>[2x]GEIQWMKSNKETGRLNINGPTRTKLEPSAFYDVFEGSKKPAVLTSKDPRLEVDFEQALFSKYVGNTLHEPDEYVTQAALHYANQLKQLDINVNKMSMEEAC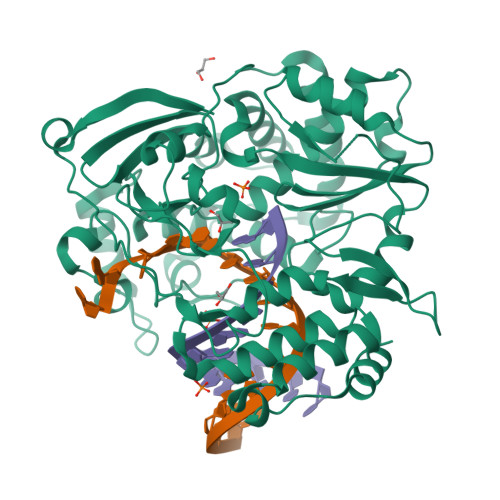YGTEYLEAIDLHTSAGYPYSALGVKKRDILDPITRDTTKMKFYMDKYGLDLPYSTYVKDELRSLDKIRKGKSRLIEASSLNDSVYLRMTFGHLYETFHANPGTVTGSAVGCNPDVFWSKLPILLPGSLFAFDYSGYDASLSPVWFRALEVVLREIGYPEEAVSLIEGINHTHHVYRNRTYCVLGGMPSGCSGTSIFNSMINNIIIRTLLIKTFKGIDLDELHMVAYGDDVLASYPFPIDCLELAKTGKEYGLTMTPADKSPCFNEVTWENATFLKRGFLPDHQFPFLIHPTMPMREIHESIRWTKDARNTQDHVRSLCLLAWHNGKEEYEKFVSTIRSVPIGRALAIPNYENLRRNWLELFHHHHHH>PRVDPRVDP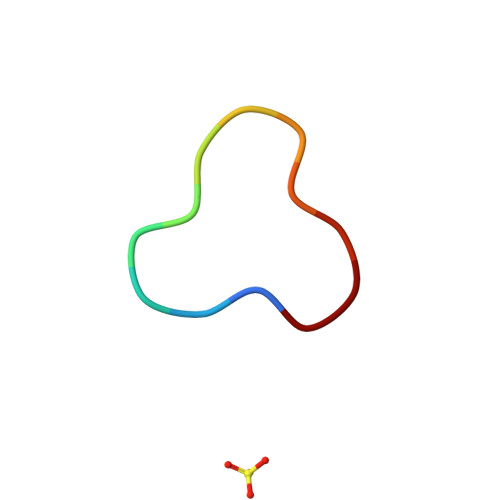RVD[2x]>GSMNDRDFMRYSRQILLDDIALDGQQK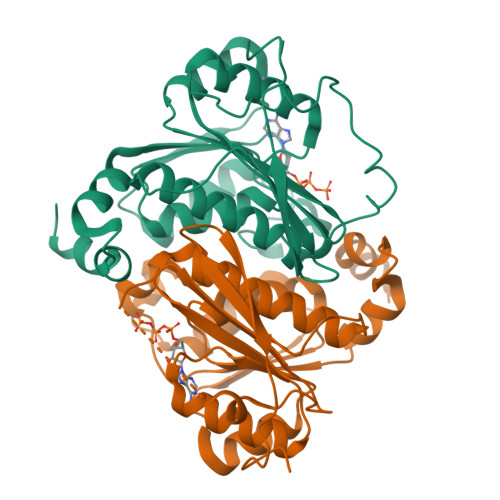LLDSQVLIIGLGGLGTPAALYLAGAGVGTLVLADDDDVHLSNLQRQILFTTEDIDRPKSQVSQQRLTQLNPDIQLTALQQRLTGEALKDAVARADVVLDCTDNMATRQEINAACVALNTPLITASAVGFGGQLMVLTPPWEQGCYRCLWPDNQEPERNCRTAGVVGPVVGVMGTLQALEAIKLLSGIETPAGELRLFDGKSSQWRSLALRRASGCPVCGGSNADPV[4x]>[2x]MEHHHHHHNKDLKGLYAALLVPF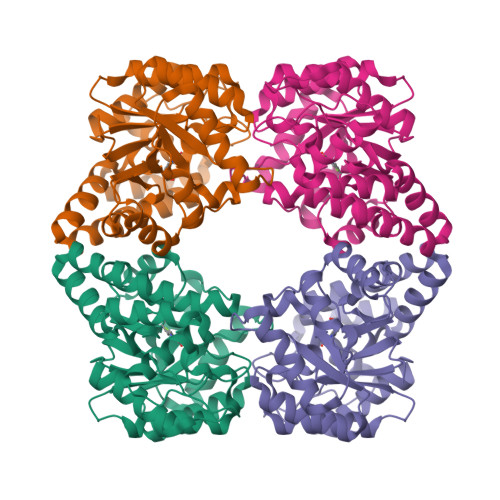DENGQVNEQGLKQIAQNAIETEELDGLYVNGSSGENFLLNTEQKKQVFKVAKEAVGDKVKLIAQVGSLDLNEAIELGKYATELGYDALSAVTPFYYPFTFEEIRDYYFDIIEATQNNMIIYAIPDLTGVNISIEQFSELFNHEKIVGVKYTAPNFFLLERIRKAFPDKLILSGFDEMLVQATISGVDGAIGSTYNVNGRRARKIFDLARQGQIQEAYQLQHDSNDIIETVLSMGIYPTLKEILRHRGIDAGLPKRPFKPFNEAHRQTLDQLIAKYDL> MDRAWFAFEAAAIPGSARHFIAPPFPVGFWARPGFGEGLDARLALAHANARRRAAAAALDNAMAAGARLEAEVDEQLRPLERQVERVAEALVVLEETARAAEEADAARAAEEAPEATAAADEGREVQIAKNDVALAYDANLSLDFLAMVYAARGAASGVLFGTWYATLQATLVAERPQVSRAIDSRDGRMSRTFMGVTTTALQACGRLYVGNRHYSALESAALCLHLVHRARQGPGAAGAAAPLGIADLLERVPEYLDALSQALAEGGRISYRYNYARVPREQLHGRYALEGHSVLAALARLRVVPGANVGANEVDGAGFVDEVNRAAAAFLGRGQNLFLGEDAPLLRATVNTITGLLLLRRLLHNGNVYGDRLRNNFQLGALVPNAPPPRGASGDAPASRSGDGNLRFLLAHYVVVA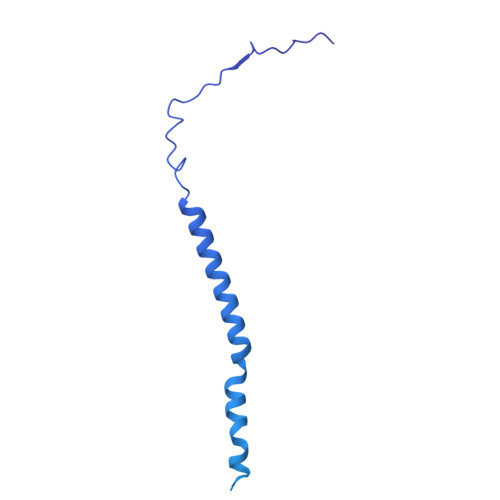YRADERTELTQLFPGLAALALDAHSIRARVQRHQLNLVRLVALELQNRQRVTAPVNEVIAAHDAVAVQYEEGLGLLLQQPHLRNAADKRLGQFGVSSDYDLLYFLCLGYIPQFAAA> SNAMALKKPGSLTIAGSGIASIGHITLETLALIKEADKIFYAVTDPATECYIQENSRGDHFDLTTFYDTNKKRYESYVQMSEVMLRDVRAGRN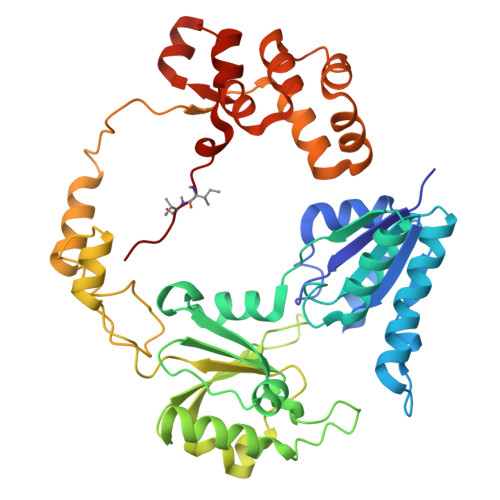VLGIFYGHPGVFVAPSHRAIAIAREEGFQAKMLPGISAEDYMFADLGFDPSTYGCMTQEATELLVRNKKLDPSIHNIIWQVGSVGVDTMVFDNGKFHLLVERLEKDFGLDHKIQHYIGAILPQSVTVKDTFAIRDLRKEEVLKQFTTTSTFYVPPRTPAPIDPKAVQALGLPATVTKGAQDWTGFQSVSPAYGPDEMRAVAALDSFVPSQEKAVVHASRAMQSLMVDLALRPALLEQYKADPVAFANTRNGLTAQEKFALGLKKPGPIFVVMRQLPSAIASGQEPSQEEIARADDATAFIIIXIVQG> MEKTEKNELVRKLIFNPQGDREASKRKIIKGNPTNIFELNEIKYSWAFDLYKLMGFTNFWIPEEIQMLEDRKQYETVLSDYEKRAYELVLSFLIALDSFQVDMLKEFGRMITAPEVEMAITAQEFQESVHAYSYQFILESVVD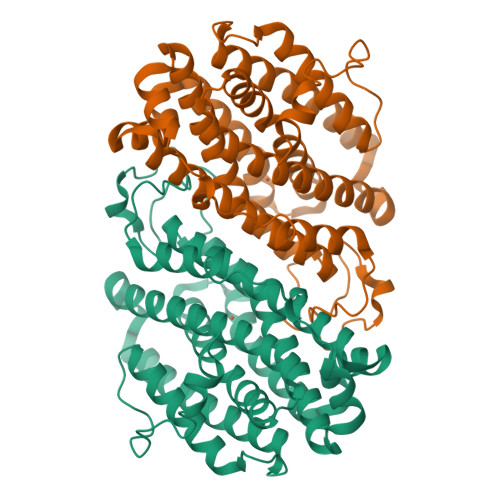PVKADEIYNYWREDERLLERNKVIAELYNEFIRKPNEENFIKATIGNYILESLYFYSGFAFFYTLGRQGKMRNTVQQIKYINRDELCHVTLFRNIINTLRKENPELFTPEIEKWIVEYFKYAVNEEIKWGQYVTQNQILGINDVLIERYIKYLGNLRITQIGFDPIYPEVTENPLKWIDEFRKINNTKTDFFQAKPQTYSKANELKW>[2x]GENGESVVVLDKYGYPILYAPEEIGEEKEYSKYEDVVIEWN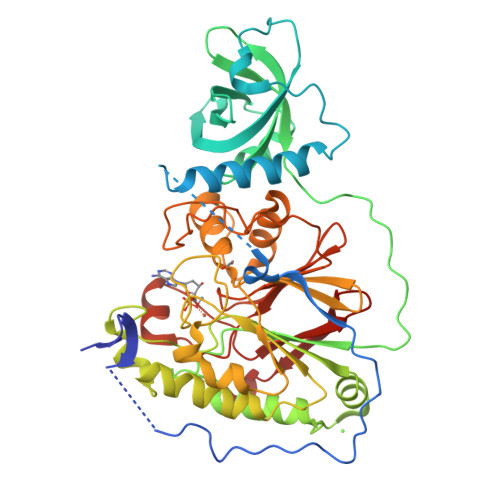PSVTPVQIEKNYEVKFDVRQVKLRPPKVKNGSGKEGEIIVEAYASLFKSRLSKLKRILRENPEISNVVDIGKLNYVSGDEEVTIIGLVNSKRETNRGLIFEVEDKTGIVKVFLPKDSEDYREAFKVLPDAVVAFKGFYSKKGIFFANKFYLPDVPLYRKQKPPLEEKVYAILISDIHVGSREFCEKAFLKFLEWLNGHVESKEEEEIVSRVKYLIIAGDVVDGIGIYPGQYSDLVIPDIFDQYEALANLLANVPEHITMFIGPGNHDAARPAIPQPEFYKEYAKPIYKLKNAIIISNPAVIRLHGRDFLIAHGRGIEDVVSFVPGLTHHKPGLPMVELLKMRHLAPTFGGKVPIAPDPEDLLVIEEVPDLVQMGHVHVYDAVVYRGVQLVNSATWQAQTEFQKMVNIVPTPAKVPVVDVESARVVKVLDFSGWC> MGLTNRLNATSNYSEYSLSVAVLADSEIENVTQLTSVTAPTGTDNENIQKLLADIKSSQNTDLTVNQSSSYLAAYKSLIAGETKAIVLNSVFENIIELEYPDYASKIKKIYTKGFTKKVEAPKTSKNQSFNIYVSGIDTYGPISSVSRSDVNILMTVNRDTKKILLTTTPRDAYVPIADGGNNQKDKLTHAGIYGVDSSIHTLENLYGVDINYYVRLNFTSFLKMIDLLGGVDVHNDQEFSALHGKFHFPVGNVHLDSEQALGFVRERYSLADGDRDRGRNQQKVIVAILQKLTSTEALKNYSTIINSLQDSIQTNVPLETM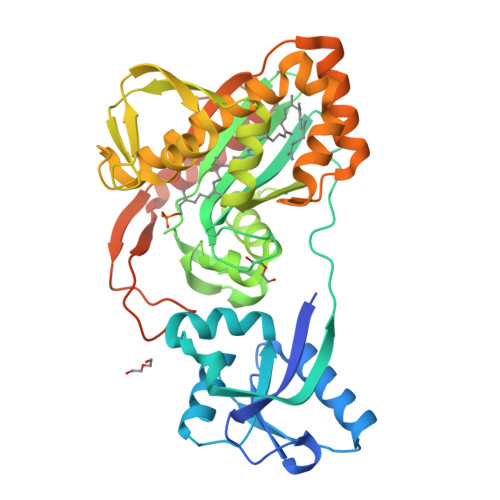INLVNAQLESGGNYKVNSQDLKGTGRMDLPSYAMPDSNLYVMEIDDSSLAVVKAAIQDVMEGRKLAAALEHHHHHH>[8x]MPHVENDGVKIYY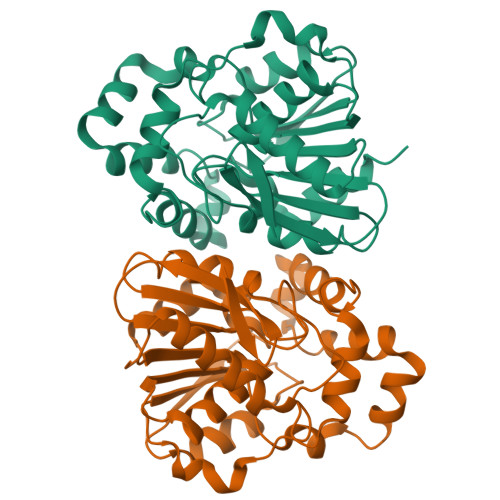DSYGEGVPIVFLHPFSTNGGIWYFQTFPFAQTNHVIVIDHRGHGRSDKPATGYSIMEHADDVVAVLDALKVDRAVFVGNSIGGMIAMQLNLDHPQRVIGNLILSSGTGLGEGMPPEAGAAFQNDYIGAFGGLLEGAVSARSKRERPEILAVMKAHFSVPSNFPKHVFDAATADPNGVFAWNIKDRLSSIQAPTLVVAGEEDLVTTVANNQLLADNIPGAELRVINDVGHFYQLERPSEFNELLRGFVAAALEHHHHHH> MIAEPLQNEIGEEVFVSPITGEIHPITDVPDQVFSGKMMGDGFAILPSEGIVVSPVRGKILNVFPTKHAIGLQSDGGREILIHFGIDTVSLKGEGFTS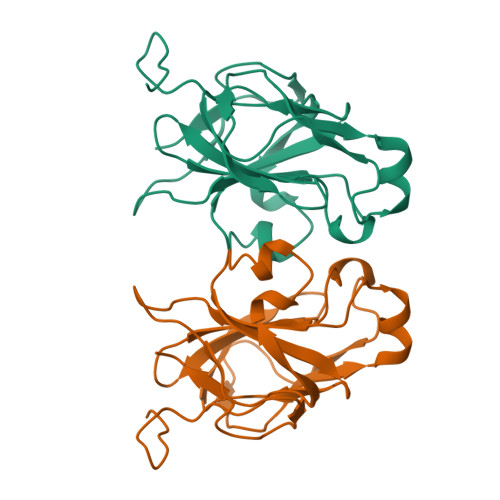FVSEGDRVEPGQKLLEVDLDAVKPNVPSLMTPIVFTNLAEGETVSIKASGSVNREQEDIVKIEK>GSHMASMTGGQQMGRGSQKPATNPVIYADAPDMSMLRVGDTYYMSSTTMHMSPGVPIMKSNDLVNWKLVNYAYDTLANIPTMNLDDGKNTYGRGSWASCLRYHEGVYYLSTFAQTTGKTYFYTTKNLEKGPWKCTEFSPAYHDHSFFFDEDGHIYMIYGNGKLFLAELKPDLSGVKPGTERVLIENASAPAGDNIMLGAEGSQLFKVNGKYYLFNITWPRGGVRTVIVHRADKITGPYEGRVVFQDRGIAQGGLVDTPDGRWFAYLFEDCGAVGRIPYLVPVEWKDGWPVLGVNGRAPAKLELPDSRGLIPGIVASDDFNRKKGERALPLVWQWNHNPDNALWSLSARKGYLRLTTGRMETSFTQAKNILTQRTIGPVCTGSVSMDVSGMKEGDFAGLSLFQRKYGQVGVKVTDGKKYIVMVNGENETPAEVEKVPLNQQVVYFKAECDFRNKVDKGYFYYSLDGSNWKAIGNVLKMQYTMPHFMGYRFALFNYATKEVGGYADFDYFKIEDKISDCRWEDICYADDKLEGHKLDIYLPDMDEPSYKVVVLIYGSAWFANNMKQAAFQVFGKSLLDKGFAVVSINHRSSGDAKFPAQINDVKAAIRFIRANAAKYKLDTSFIGITGFSSGGHLASLAGTTNGVKSYTIGAKTVDLEGNVGLYPSFSSRVDAVVN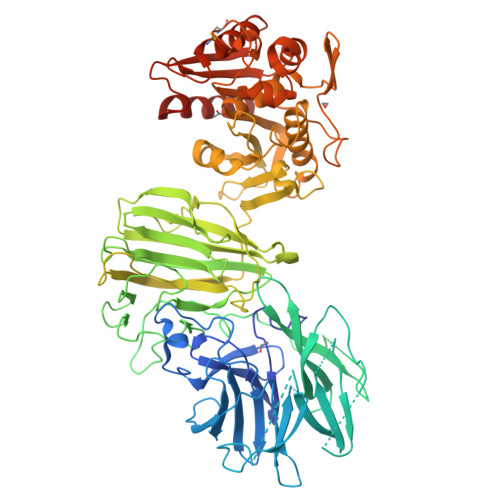WFGPIDMTRMENCNTTKGANSPEAALIGGVPADNLDMLALLNPITYIDKNDPKFIVIHGEADTVVPNCQSIFFSEALRAQGRLEEFISVPGGQHGPVTFNENTLKKMIDFFAREAGIYRDLNRIRPIKCDDIK[4x]> TN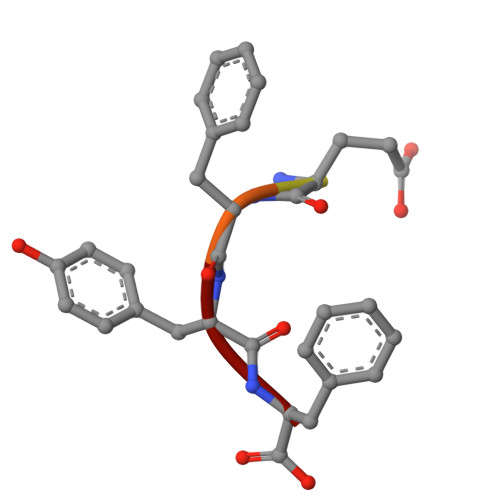EFYF2-{(S)-(3-{[4-(dimethylamino)butanoyl]amino}phenyl)[2-(piperidin-1-yl)ethoxy]methyl}thieno[3,2-b]pyridine-7-carboxylic 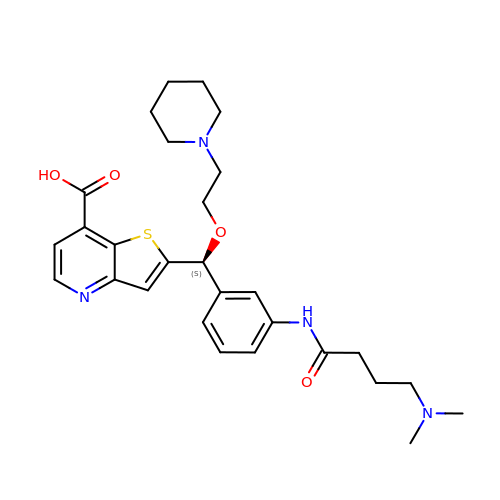acid | C28 H36 N4 O4 S | GTUZDQNWYGEDTB-SANMLTNESA-N>DLIVNLTDSKGTCLYAEWEMNFTITYETTNQTNKTITIAVPDKATHDGSSCGDDRNSAKIMIQFGFAVSWAVNFTKEASHYSIHDIVLSYNTSDSTVFPGAVAKGVHTVKNPENFKVPLDVIFKCNSVLTYNLTPVVQKYWGIHLQAFVQNGTVSK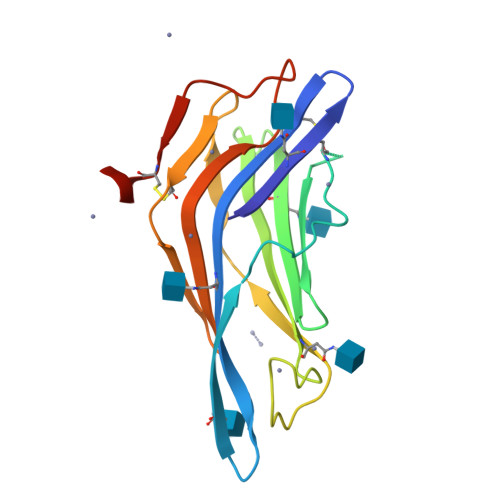NEQVCEEDQGSSL[2x]> GVTFDDGAYTGIREINFEYNSETAIGGLRVTYDLNGMPFVAEDHKSFITGFKPVKISLEFPSEYIVEVSGYVGKVEGYTVIRSLTFKTNKQTYGPYGVTNGTPFSLPIENGLIVGFKGSIGYWLDYFSIYLSL;> GRNGKSQ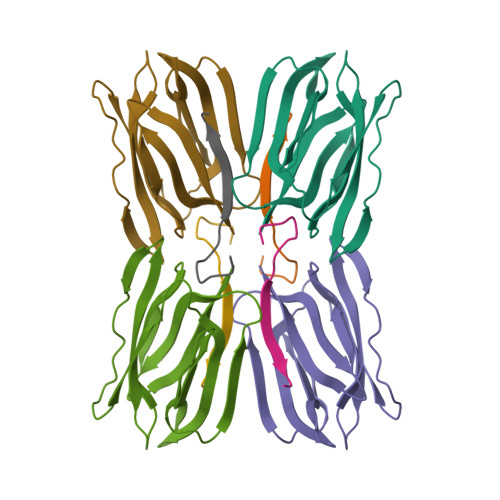SIIVGPWGD> MKHHHHHHMKQNSPLDEENLTQENQDRGTHVDRGLASANVDFAFSLYKQLVLKAPDKNVIFSPLSISTALAFLSLGAHNTTLTEILKGLKFNLTETSEAEIHQSFQHLLRTLNQ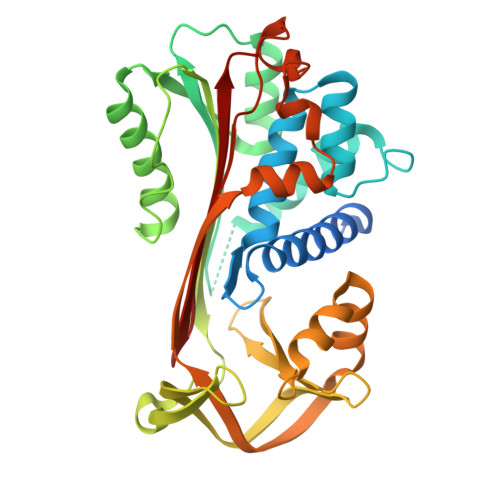SSDELQLSMGNAMFVKEQLSLLDRFTEDAKRLYGSEAFATDFQDSAAAKKLINDYVKNGTRGKITDLIKDLDSQTMMVLVNYIFFKAKFEMPFDPQDTHQSRFYLSKKKYVMVPMMSLHHLTIPYFRDEELSCTVVQLNYTGNASALFILPDQDKMEEVEAMLSQETLSRFFDSLEFREIGELYLPKFSISRDYNLNDILLQLGIEEAFTSKADLSGITGARNLAVSQVVHKAVLDVFEEGTEASAATALFIPLS> GGGRGENFMDIECFMVLNPSQQLAIAVLSLTLGTFTVLENLLVLCVILHSRSLRCRPSYHFIGSLAVADLLGSVIFVYSFIDFHVFHRKDSRNVFLFKLGGVTASFTASVGSLFLAAIDRYISIHRPLAYKRIVTRPKAVVAFCLMWTIAIVIAVLPLLGWNCEKLQSVCSDIFPHIDKTYLMFWIGVVSVLLLFIVYAYMYILWKAHSHAVAKALIVYGSTTGNTEYTAETIARELADAGYEVDSRDAASV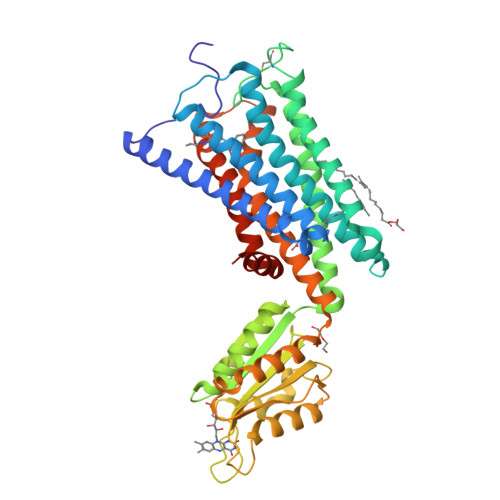EAGGLFEGFDLVLLGCSTWGDDSIELQDDFIPLFDSLEETGAQGRKVACFGCGDSSWEYFCGAVDAIEEKLKNLGAEIVQDGLRIDGDPRAARDDIVGWAHDVRGAIPDQARMDIELAKTLVLILVVLIICWGPLLAIMVYDVFGKMNKLIKTVFAFCSMLCLLNSTVNPIIYALRSKDLRHAFRSMFPSHHHHHHHHHH> QGIREVILCKDQDGKIGLRLKSVDNGIFVQLVQANSPASLVGLRFGDQVLQINGENCAGWSSDKAHKVLKQAFGEKITMTIRDRPFERTVTMHKDSSGHVGFIFKSGKITSIVKDSSAARNGLLTDHHICEINGQNVIGLKDAQIADILSTA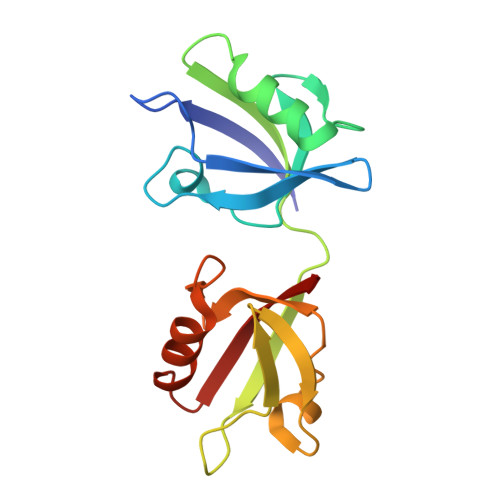GTVVTITIMPA>HCHQQLNSLPTMEGPPTFNPPVPYFGRLQGGLTARRTIIIKGYVPPTGKSFAINFKVGSSGDIALHINPRMGNGTVVRNSLLNGSWGSEEKKITHNPFGPGQFFDLSIRCGLDRFKVYANGQHLFDFAHRLSAFQR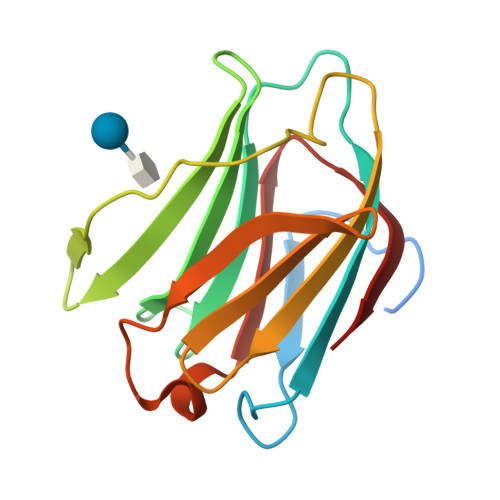VDTLEIQGDVTLSYVQI[4x]> XL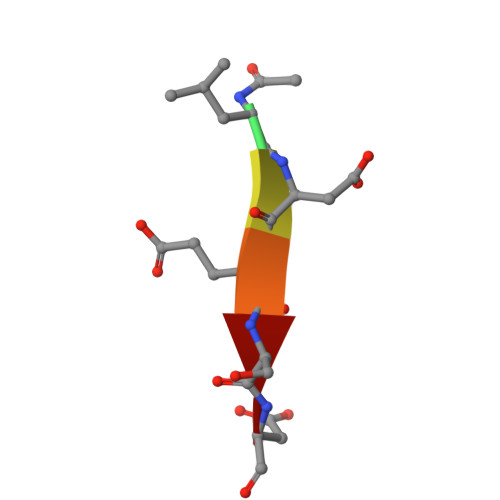DESD> MPLKFPEMFLFGTATSSHQIEGNNRWNDWWYYEQIGKLPYRSGKACNHWELYRDDIQLMTSLGYNAYRFSIEWSRLFPEENKFNEDAFMKYREIIDLLLTRGITPLVTLHHFTSPLWFMKKGGFLREENLKHWEKYIEKVAELLEKVKLVATFNEPMVYVMMGYLTAYWPPFIRSPFKAFKVAANLLKAHAIAYELLHGKFKVGIVKNIP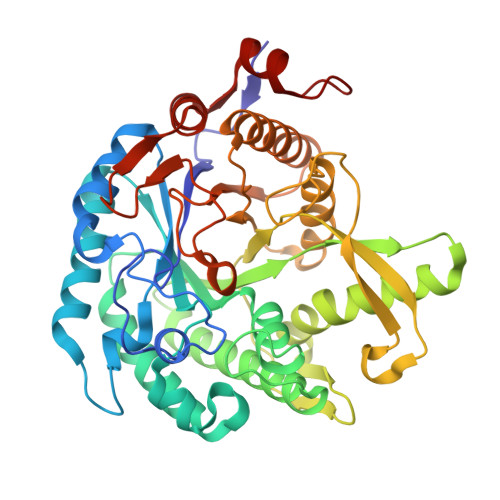IILPASDKERDRKAAEKADNLFNWHFLDAIWSGKYRGVFKTYRIPQSDADFIGVNYYTASEVRHTWNPLKFFFEVKLADISERKTQMGWSVYPKGIYMALKKASRYGRPLYITENGIATLDDEWRVEFIIQHLQYVHKAIEDGLDVRGYFYWSFMDNYEWKEGFGPRFGLVEVDYQTFERRPRKSAYVYGEIARSKEIKDELLKRYGLPELQL(2S)-2-butyl-6,7-bis(chloranyl)-2-cyclopentyl-5-[3-(1H-1,2,3,4-tetrazol-5-yl)propoxy]-3H-inden-1-one | C22 H28 Cl2 N4 O2 | 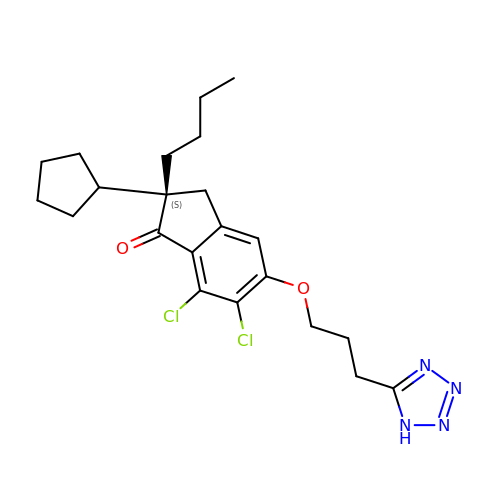ZGKIUQSJMFBDGB-QFIPXVFZSA-N>[3x]ATAAEIAALPRQKVELVDPPFVHAHSQVAEGGPKVVEFTMVIEEKKIVIDDAGTEVHAMAFNGTVPGPLMVVHQDDYLELTLINPETNTLMHNIDFHAATGAL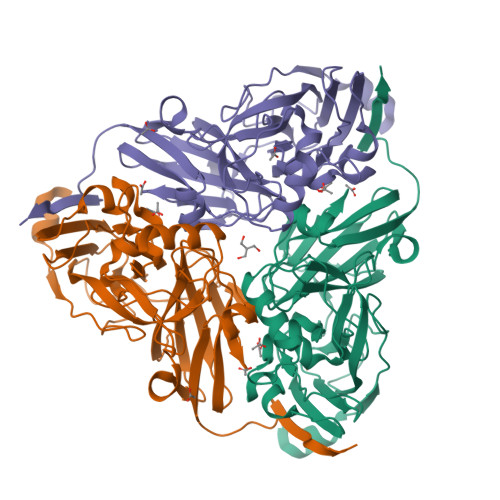GGGGLTEINPGEKTILRFKATKPGVFVYHCAPPGMVPWHVVSGMNGAIMVLPREGLHDGKGKALTYDKIYYVGEQDFYVPRDENGKYKKYEAPGDAYEDTVKVMRTLTPTHVVFNGAVGALTGDKAMTAAVGEKVLIVHSQANRDTRPHLIGGHGDYVWATGKFNTPPDVDQETWFIPGGAAGAAFYTFQQPGIYAYVNHNLIEAFELGAAAHFKVTGEWNDDLMTSVLAPSGTIEGR>MVKWRTLVHNGVALPPPYQPKGLSIKIRGETVKLDPLQEEMAYAWALKKDTPYVQDPVFQKNFLTDFLKTFNGRFQDVTINEIDFSEVYEYVERERQLKADKEYRKKISAERKRLREELKARYGWAEMDGKRFEIANWMVEPPGIFMGRGNHPLRGRWKPRVYEEDITLNLGEDAPVPPGNWGQIVHDHDSMWLARWDDKLTGKEKYVWLSDTADIKQKRDKSKYDKAEMLENHIDRVREKIFKGLRSKEPKMREIALACYLIDRLAMRVGDEKDPDEADTVGATTLRVEHVKLLEDRIEFDFLGKDSVRWQKSIDLRNEPPEVRQVFEELLEGKKEGDQIFQNINSRHVNRFLGKIVKGLTAKVFRTYIATKIVKDFLAAIPREKVTSQEKFIYYAKLANLKAAEALNHKRAPPKNWEQSIQKKEE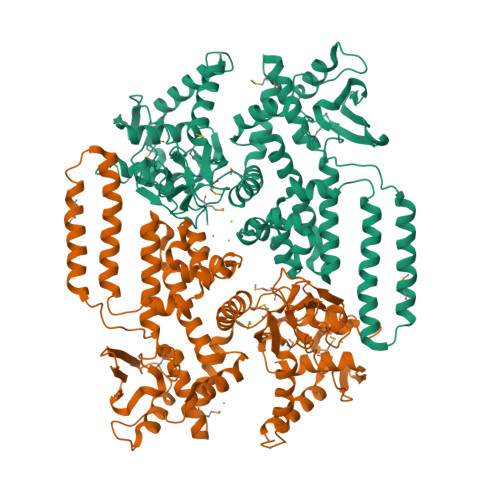RVKKLMQQLREAESEKKKARIAERLEKAELNLDLAVKVRDYNLATSLRNYIDPRVYKAWGRYTGYEWRKIYTASLLRKFKWVEKASVKHVLQYFAEKLAKDVDKGMQVKAAV[2x]>[3x]MNPAHLLVLSAVCVSLLGASSIPPQPL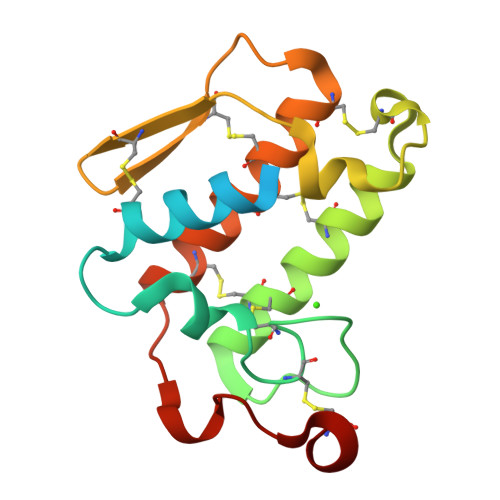HLIQFGNMIQCTVPGFLSWIKYADYGCYCGAGGSGTPVDKLDRCCQVHDNCYTQAQKLPACSSIMDSPYVKIYSYDCSERTVTCKADNDECAAFICNCDRVAAHCFAASPYNNNNYNIDTTTRC> DCPPDWSSYEGHCYRFFKEWMHWDDAEEFCTEQQTGAHLVSFQSKEEADFVRSLTSEMLKGDVVWIGLSDVWNKCRFEWTDGMEFDYDDYYLIAEYEC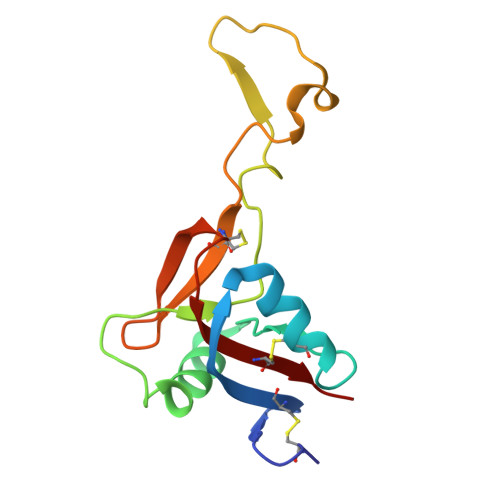VASKPTNNKWWIIPCTRFKNFVCEFQA>[2x]G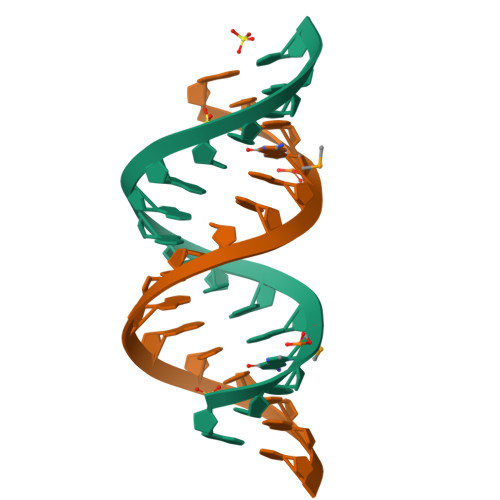CAGAGUUAAAUCUGC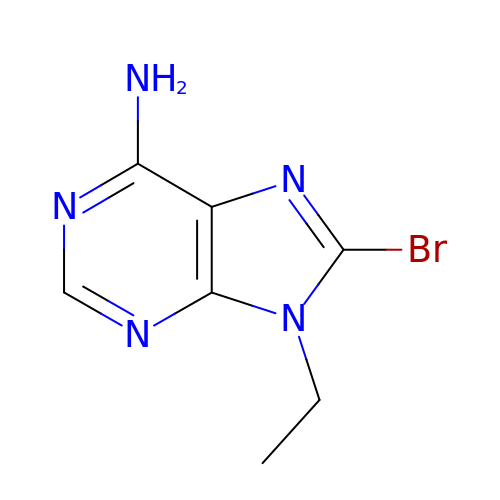8-bromanyl-9-ethyl-purin-6-amine | C7 H8 Br N5 | GACDSQLJMZANKT-UHFFFAOYSA-N>[8x]MPHVENASETYIPGRLDGKVALVTGSGRGIGAAVAVHLGRLGAKVVVNYANSTKDAEKVVSEIKALGSDAIAIKADIRQVPEIVKLFDQAVAHFGHLDIAVSNSGVVSFGHLKDVTEEEFDRVFSLNTRGQFFVAREAYRHLTEGGRIVLTSSNTSKDFSVPKHSLYSGSKGAVDSFVRIFSKDCGDKK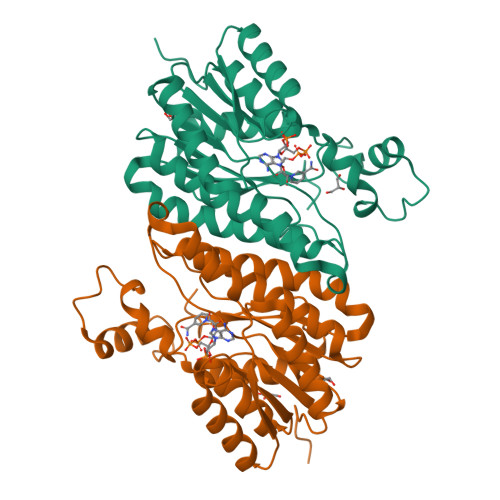ITVNAVAPGGTVTDMFHEVSHHYIPNGTSYTAEQRQQMAAHASPLHRNGWPQDVANVVGFLVSKEGEWVNGKVLTLDGGAA>[12x]HCDLPCGVYDPAQARIEAESVKAIQEKMAANDDL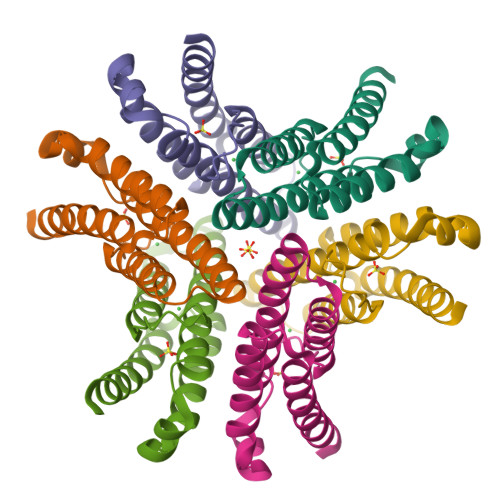HFQIRATVIKEQRAELAKHHLDVLWSDYFKPPHFESYPELHTLVNEAVKALSAAKASTDPATGQKALDYIAQIDKIFWETKKA> SIFDDDMDDIF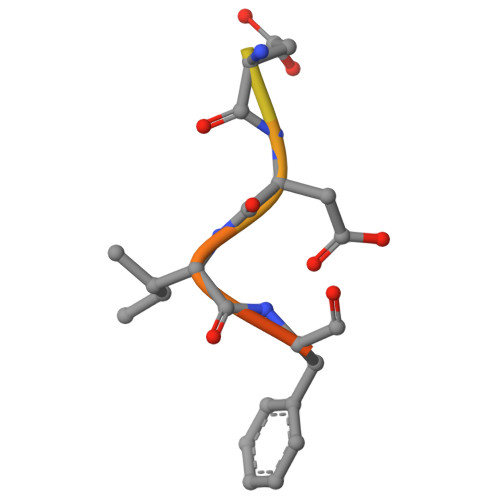SSG> GDPHMSTFIFPGDSFPVDPTTPVKLGPGIYCDPNTQEIRPVNTGVLHVSAKGKSGVQTAYIDYSSKRYIPSVNDFVIGVIIGTFSDSYKVSLQNFSSSVSLSYMAFPNASKKNRPTLQVGDLVYARVCTAEKELEAEIECFDSTTGRDAGFGILEDGMIIDVNLNFARQLLFNNDFPLLKVLAAHTKFEVAIGLNGKIWVKCEELSNTLACYRTIMECCQKNDTAAFKDIAKRQFK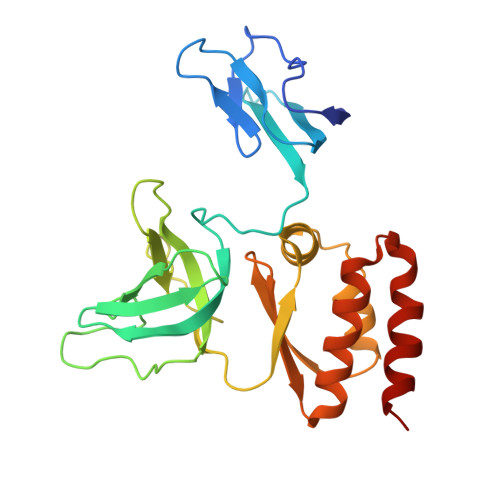EILTVKEE> ETRYEKFLRQHVD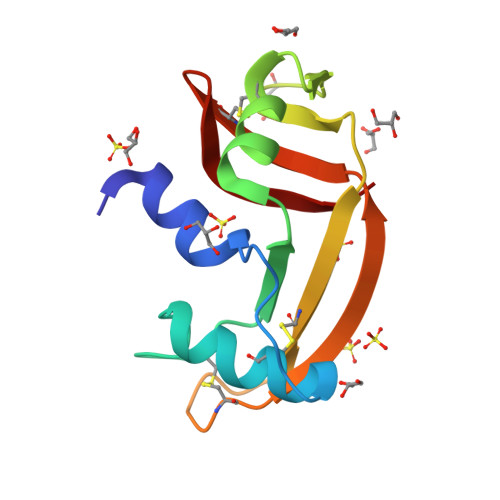YPRTAAPDTRTYCNQMMQRRGMTLPVCKFTNTFVHASAASITTICGPGGAPAGGNLRDSTASFALTTCRLQGGSQRPPCNYNGGTSTQRIRIACDGGLPVHYDRAI> DPDTAVTNKQSFSTDVIYQVFTDRFLDGNPSNNPTGAAYDATCSNLKLYCGGDWQGLINKINDNYFSDLGVTALWISQPVENIFATINYSGVTNTAYHGYWARDFKKTNPYFGTMADFQNLITTAHAKGIKIVIDFAPNHTSPAMETDTSFAENGRLYDNGTLVGGYTNDTNG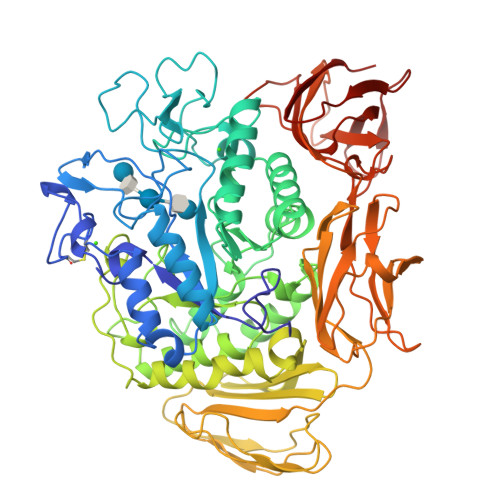YFHHNGGSDFSSLENGIYKNLYDLADFNHNNATIDKYFKDAIKLWLDMGVDGIRVDAVKHMPLGWQKSWMSSIYAHKPVFTFGAWFLGSAASDADNTDFANKSGMSLLDFRFNSAVRNVFRDNTSNMYALDSMINSTATDYNQVNDQVTFIDNHDMDRFKTSAVNNRRLEQALAFTLTSRGVPAIYYGTEQYLTGNGDPDNRAKMPSFSKSTTAFNVISKLAPLRKSNPAIAYGSTQQRWINNDVYVYERKFGKSVAVVAVNRNLSTSASITGLSTSLPTGSYTDVLGGVLNGNNITSTNGSINNFTLAAGATAVWQYTTAETTPTIGHVGPVMGKPGNVVTIDGRGFGSTKGTVYFGTTAVTGAAITSWEDTQIKVTIPSVAAGNYAVKVAASGVNSNAYNNFTILTGDQVTVRFVVNNASTTLGQNLYLTGNVAELGNWSTGSTAIGPAFNQVIHQYPTWYYDVSVPAGKQLEFKFFKKNGSTITWESGSNHTFTTPASGTATVTVNWQ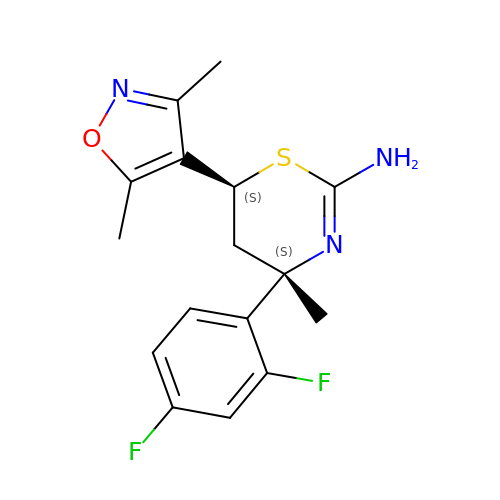(4~{S},6~{S})-4-[2,4-bis(fluoranyl)phenyl]-6-(3,5-dimethyl-1,2-oxazol-4-yl)-4-methyl-5,6-dihydro-1,3-thiazin-2-amine | C16 H17 F2 N3 O S | XCTPNVXKKHOANI-BBRMVZONSA-N> MKKGHHHHHHGSERTGTQPLGVQGLTEEQRMMIRELMDAQMKTFDTTFSHFKNFRLPGVLSSGCELPESLQAPSREEAAKWSQVRKDLCSLKVSLQLRGEDGSVWNYKPPADSGGKEIFSLLPHMADMSTYMFKGIISFAKVISYFRDLPIEDQISLLKGAAFELCQLRFNTVFNAETGTWECGRLSYCLEDTAGGFQQLLLEPML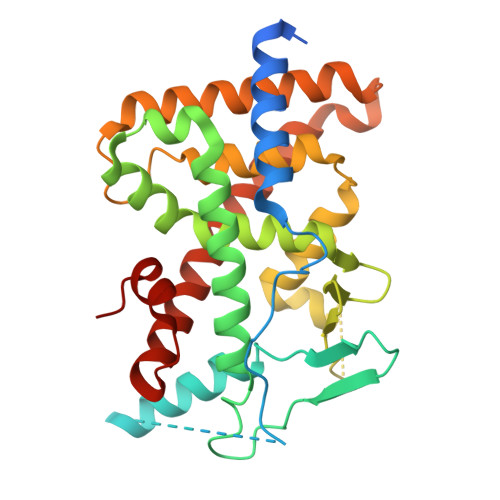KFHYMLKKLQLHEEEYVLMQAISLFSPDRPGVLQHRVVDQLQEQFAITLKSYIECNRPQPAHRFLFLKIMAMLTELRSINAQHTQRLLRIQDIHPFATPLMQELFGIT>[4x]MRRHGFSLLELLLASVLMGSLLLVVLALENSSATLRERERARGRLADELSLTATVLARELYTVGYRLTGQALVLSPSSQGDGVQGWFLCEAGMEEICGESMGEVRGTGYEVNQGALRWGACKGEGCAPLPNNPVLGGDEVQVEAFRVAYLEGGTWKRQAQAVNLRPEGASPKVSALALYLLASVPVRGGAPAFTPGSTLSYPPGLTSSLLELPGAPNDGRLRAEKLWIVQTPNLAR

Type IV pili (T4P)1 are long, surface-exposed filaments which extend from the surfaces of bacterial cells. T4P are composed of both major and minor pilin components, although major pilins comprise the majority of the pilin subunits within each fibre. We identified a cluster of type IV pilin-like genes within the T. thermophilus HB8 genome, using the program PilFind. Three of the remaining six, TTHA1218, TTHA1219 and TTHA1222, yielded crystals of truncated forms which enabled us to solve their structures (designated here as Tt121836-123, Tt121933-236 and Tt122238-123).

Tt121933-236 crystallized in two different crystal forms; the higher resolution form, at 1.85 Å resolution in spacegroup P21, has four molecules in the asymmetric unit, arranged as a dimer of dimers. The interfaces between monomers were analyzed by PISA, which revealed that the interface areas between chains A and B, and its equivalent between C and D, were substantial, with a mean of 1488 Å2 (the next largest interface area was 439 Å2). The CSS score for both interfaces was 1.0, suggesting that Tt121933-236 forms a dimer in solution. The monomer-monomer interface is dominated by the helix-helix interaction across the non-crystallographic 2-fold symmetry axis. The second crystal form, in spacegroup C2, has a dimer in the asymmetric unit; crucially, the interface between the A and B chain dimer is preserved in this crystal form, providing further evidence that this dimer is not a crystallization artifact. Formation of a dimer in solution by Tt121933-236 was investigated by SEC, which showed elution peaks for both monomer and dimer, as well as a third peak in the void volume, which appeared to be associated with contaminants in the preparation. Tt121933-236 forms a more complex fold topology than XcpW and the related T2SS pseudopilins, with two main differences. First, two additional β-strands, β8 and β9, are inserted into the variable β-sheet, which extend this structural feature into the same spatial location occupied by the short α2 helix in XcpW. Second, Tt121933-236 contains a long loop, from residue 184 in β10 to 221 in β11, which folds back over the external surface of the conserved sheet (marked in orange in Figs4c & d). Tt121933-236 is also stabilized by two disulphide bonds, between β2/β3, and β4/β5; both lie within the variable β-sheet.> SNLGL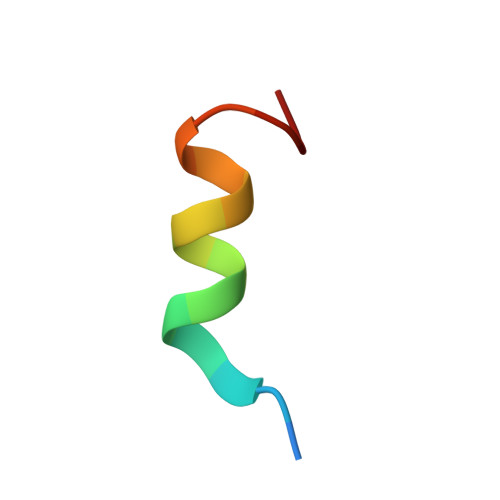EDIIRKALMGSF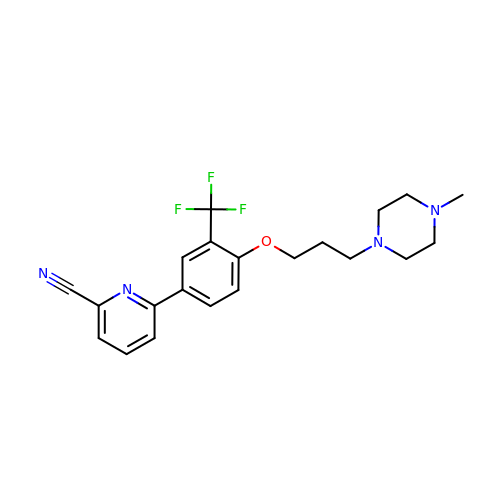6-{4-[3-(4-methylpiperazin-1-yl)propoxy]-3-(trifluoromethyl)phenyl}pyridine-2-carbonitrile | C21 H23 F3 N4 O | CWICZCHZPOSFKO-UHFFFAOYSA-N> MFKIVYPNA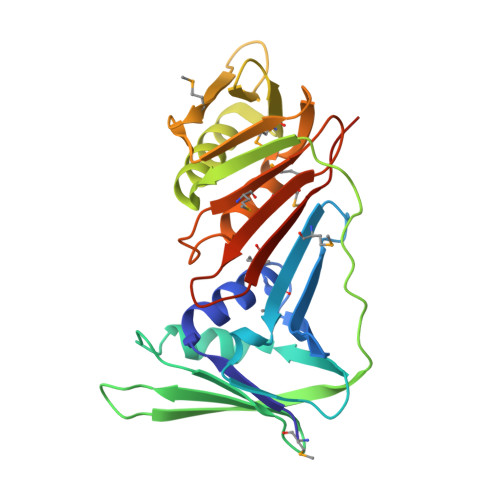KDFFSFINSITNVTDSIILNFTEDGIFSRHLTEDKVLMAIMRIPKDVLSEYSIDSPTSVKLDVSSVKKILSKASSKKATIELTETDSGLKIIIRDEKSGAKSTIYIKAEKGQVEQLTEPKVNLAVNFTTDESVLNVIAADVTLVGEEMRISTEEDKIKIEAGEEGKRYVAFLMKDKPLKELSIDTSASSSYSAEMFKDAVKGLRGFSAPTMVSFGENLPMKIDVEAVSGGHMIFWIAPRLLEHHHHHH> MRLPDPYTNPELSGLGFESVNLIDNDPVIRDELPNGKVNEVKVSAQYWG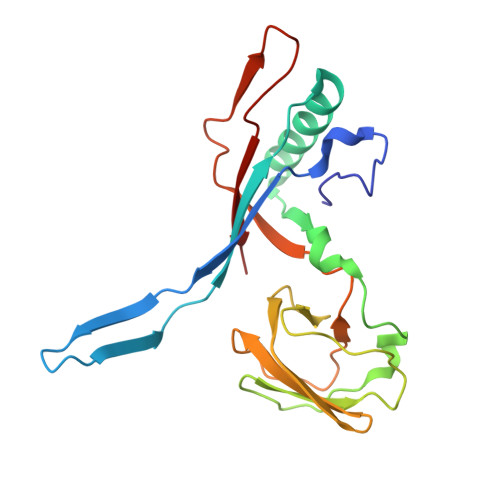INISYPELFPDEYSVLDAFILEYKRTGGYIDVILPQYEAFRVRGNTNLVNIPAGQKGSNITMDTQGVLTGIPKPGDLFKLSNHPKVYKITSFNRSGNSWSINVYPDLFITTTGAEKPVFNGILFRTKLMNGDAFGSTLNNNGTYSGISLNLRESL> MLAGVKKDIEKLYEAVPQLSNVFKIEDKIGEGTFSSVYLATAQLQVGPEEKIALKHLIPTSHPIRIAAELQCLTVAGGQDNVMGVKYCFRKNDHVVIAMPYLEHESFLDILNSLSFQEVREYMLNLFKALKRIHQFGIVHRDVKPSNFLYNRRLKKYALVD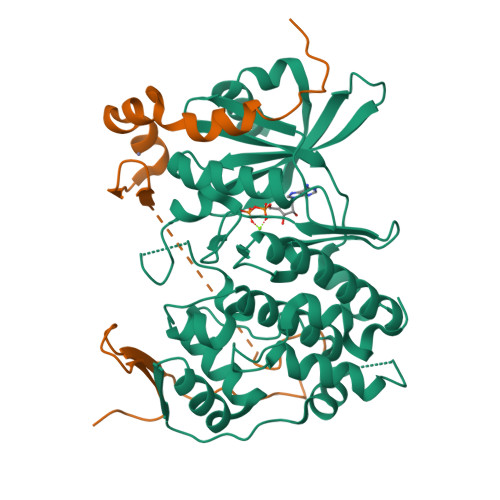FGLAQGTHDTKIELLKFVQSEAQQERCSQNKCSICLSRRQQVAPRAGTPGFRAPEVLTKCPNQTTAIDMWSAGVIFLSLLSGRYPFYKASDDLTALAQIMTIRGSRETIQAAKTFGKSILCSKEVPAQDLRKLCERLRGMDSSTPKLTSDIQGHATNLEGWNEVPDEAYDLLDKLLDLNPASRITAEEALLHPFFKDMSL;> GPGTRTGRLKKPFVKVEDMSQLYRPFYLQLTNMPFINYSIQKPCSPFDVDKPSSMQKQTQVKLRIQTDGDKYGGTSIQLQLKEKKKKGYCECCLQKYEDLETHLLSEQHRNFAQSNQYQVVDDIVSKLVFDFVEYEKDTPKKKR>MQDYTVHIVDDEEPVRKSLAFMLTM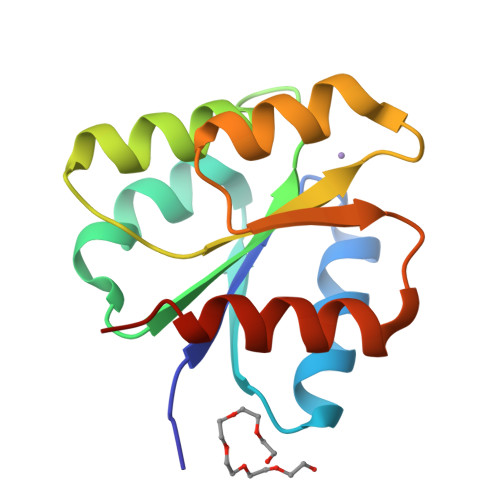NGFAVKMHQSAEAFLAFAPDVRNGVLVTDLRMPDMSGVELLRNLGDLKINIPSIVITGHGDVPMAVEAMKAGAVDFIEKPFEDTVIIEAIERASEHLVALE[2x]> APTLEINTITFDVGNATINK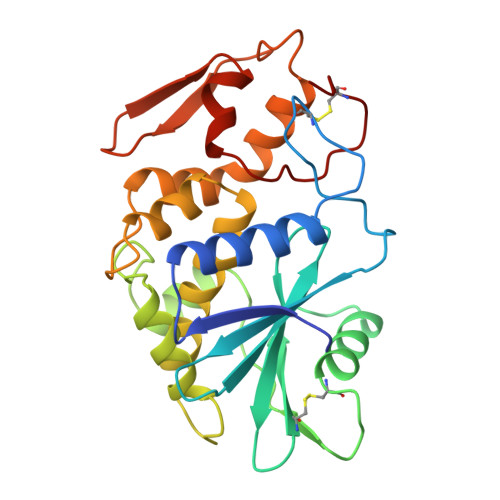YATFMKSIHNQAKDPTLKCYGIPMLPNTNLTPKYLLVTLQDSSLKTITLMLKRNNLYVMGYADTYNGKCRYHIFKDISNTTERNDVMTTLCPNPSSRVGKNINYDSSYPALEKKVGRPRSQVQLGIQILNSGIGKIYGVDSFTEKTEAEFLLVAIQMVSEAARFKYIENQVKTNFNRAFYPNAKVLNLEESWGKISTAIHNAKNGALTSPLELKNANGSKWIVLRVDDIEPDVGLLKYVNGTCQAT> GPQSEPELKLESVVIVSRHGVRAPTKATQLMQDVTPDAWPTWPVKLGWLTPRGGELIAYLGHYQRQRLVADGLLAKKGCPQSGQVAIIADVDERTRKTGEAFAAGLAPDCAITVHTQADTSSPDPLFNPLKTGVCQLDNANVTDAILSRAGGSIADFTGHRQTAFRELERVLNFPQSNLCLKREKQDESCSLTQALPSELKVSADNVSLTGAVSLASMLTEIFLLQQAQGMPEPGWGRITDSHQWNTLLSLHNAQFYLLQRTPEVARSRATPLLDLIKTALTPHPPQKQAYGVTLPTSVLFIAGHETNLANLGGALELNWTLPGQPDNTPPGGELVFERWRRLSDNSQWIQVSLVFQTLQQMRDKTPLSLNTPPGEVKLTLAGCEERNAQGMCSLAGFTQIVNEARIPACS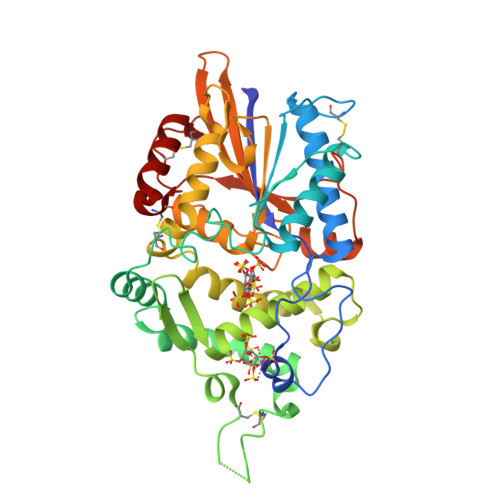L> MHNHNHNHNHNHNGGENLYFQGASLTEIEHLVQSVCKSYRETCQLRLEDLLRQRSNIFSREEVTGYQRKSMWEMWERCAHHLTEAIQYVVEFAKRLSGFMELCQNDQIVLLKAGAMEVVLVRMCRAYNADNRTVFFEGKYGGMELFRALGCSELISSIFDFSHSLSALHFSEDEIALYTALVLINAHRPGLQEKRKVEQLQYNLELAFHHHLCKTHRQSILAKLPPKGKLRS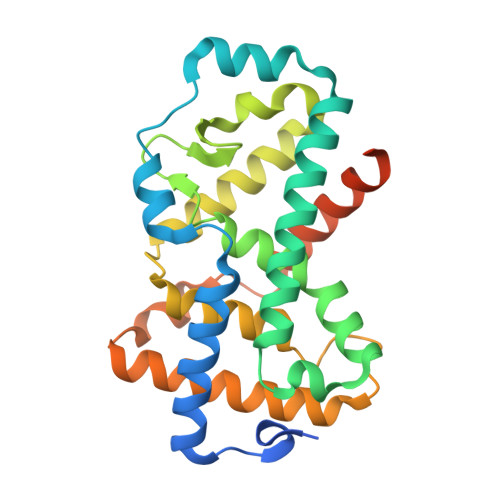LCSQHVERLQIFQHLHPIVVQAAFPPLYKELFS>MPIHNLNHVNMFLQVIASGSISSAARILRKSHTAVSSAVSNLEIDLCVELVRRDGYKVEPTEQALRLIPYMRSLLNYQQLIGDIAFNLNKGPRNLRVLLDTAIPPSFCDTVSSVLLDDFNMVSLIRTSPADSLATIKQDNAEIDIAITIDEELKISRFNQCVLGYTKAFVVAHPQHPLCNASLHSIASLANYRQISLGSRSGQHSNLLRPVSDKVLFVENFDDMLRLVEAGVGWGIAPHYFVEERLRNGTLAVLSELYEPGGIDTKVYCYYNTALESERSFLRFLESARQRLRQLGRQRFDDAPAWQPSIVETAQRRSG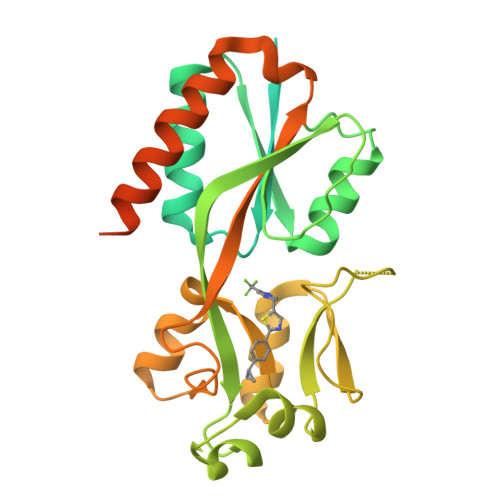PKALAYRQRAAPE[2x]>[2x]MGQNMEIDNFLKIER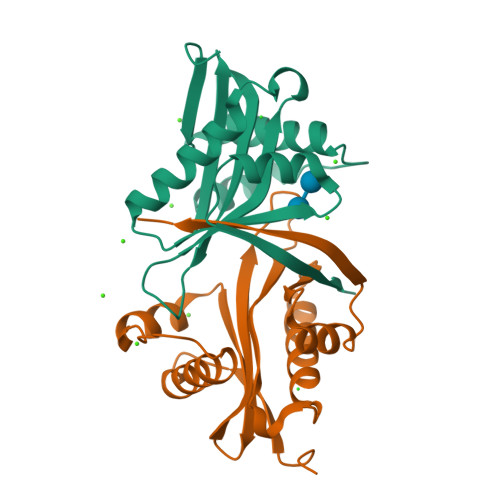LAENDLPKFIQLIRLFEAVFEMKNFSIPDSEHLQKLLNQNNFYVFVALLENKIVGGLTSYVLEQYYSEKPLAYIYDLAVDTNWQRQGIGKKLITATNQFYTEKGFEEVFVQADKVDDYALDFYRSTKPTAEEQVVHFYYTLK>GPAFEFAVAMMKRNSSTVKTEYGEFTMLGIYDKWAVLPRHAKPGPTILMNDQEVSVLDAKELVDKD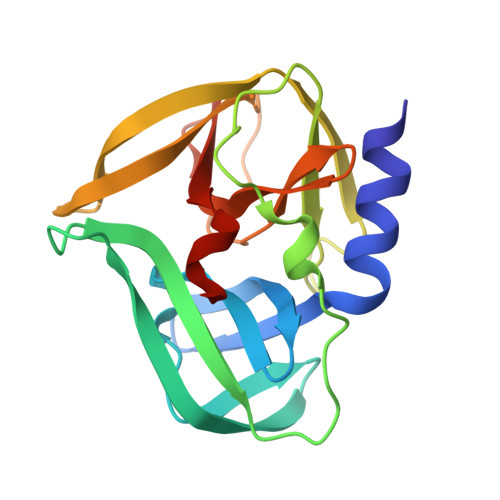GTNLELTLLKLNRNEKFRDIRGFLAKEEVEVNEAVLAINTSKFPNMYIPVGQVTDYGFLNLGGTPTKRMLMYNFPTRAGQCGGVLMSTGKVLGIHVGGNGHQGFSAALLKHYFNDEQ[2x]>GPELMVISRAEIYWADLGPPSGSQPAKRRPVLVIQSDPYNASRLATVIAAVITSNTALAAMPGNVFLPATTTRLPRDSVVNVTAIVTLNKTDLTDRVGEVPASLMHEVD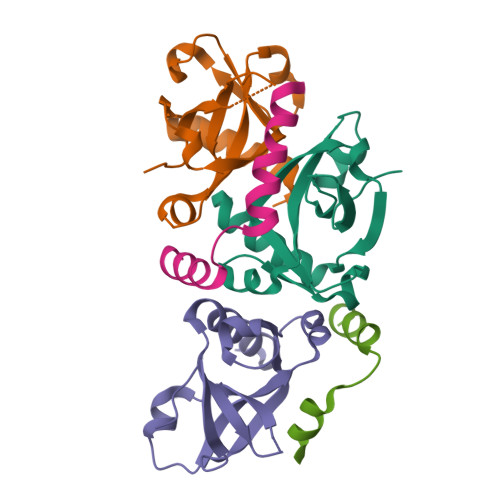RGLRRVLDL[3x];>[2x]LTGQIDRALESIHGTDEAEALAVANAYRVLETMDDEW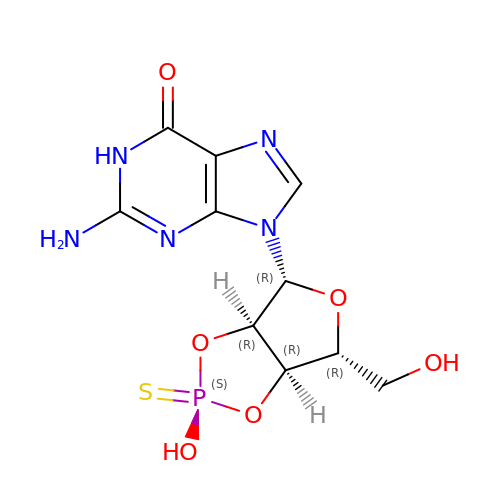GUANOSINE-2',3'-CYCLOPHOSPHOROTHIOATE | C10 H12 N5 O6 P S | QZEROIIFJLCOOE-FHIGPPGSSA-N>PPGPPGPPGPQGPKGDKGDPGPPGPPG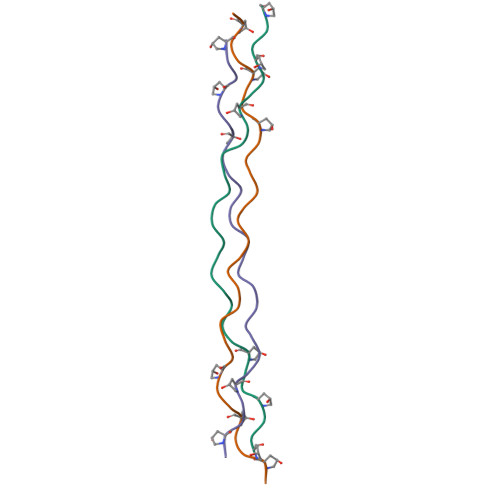PPG[3x]Serine hydroxymethyltransferase (SHMT) reversibly interconverts serine and tetrahydrofolate (THF) into glycine and 5,10-methylene-THF (5,10-meTHF). Next, we have obtained high resolution crystal structures of AtSHMT2 complexed with MTX and PTX, as well as of AtSHMT4-MTX complex. For clarity, in this work we divide THF, MTX, and PTX molecules into three moieties: (i) pteridine or its mimic (P-moiety); (ii) benzoyl (B-moiety); and (iii) glutamate (E-moiety).

Soaking crystals of AtSHMT2 with PTX and serine revealed two distinct forms, resembling situation observed for AtSHMT2-MTX complex. External PLP-Ser aldimine state (EA-type) is seen in chains B and C (PTX was not placed in chain A as suggested by poor Polder map coefficients). Internal aldimine + free serine state (IA-type) is present in chain D. In the EA-type of binding (Chain B), a direct H-bond binds exocyclic N2 of PTX to backbone O of Leu172. Water-mediated interactions involve each of the five heteroatoms in the P-moiety. Importantly, there is no π-stacking interaction involving PTX. Hydrophobic environment is ensured mostly by side chains of Leu172, Leu178, and Ile189 adjacent to PTX B-moiety. The carboxyl group (at Cα) forms a salt bridge with Nζ of Lys187. In the IA-pose (Chain D), PTX forms fewer H-bonds. Another feature that likely explains higher inhibitory efficiency of PTX against SHMTs is that it is able to bind deeper inside the cavity.

>SNAEKSRSSWIKQLNASLDEIDPEVADIIELEKARQWKGFELIPSENFTSLSVMQAVGSVMTNKYSEGYPGARYYGGNEYIDMAETLCQKRALEAFQLDPSKWGVNVQSLSGSPANFQVYTALLKPHERIMALDLPHGGHLSHGYQTDTKKISAVSIFFETMPYRLDENTGYIDYDQLEKSAVLFRPKLIVAGASAYARLYDYARIRKVCNKQKAVMLADMAHISGLVAAGVIPSPFEYADVVTTTTHKSLRGPRGAMIFFRKGLKEINKQGKEVMYDYEDRINQAVFPGLQGGPHNHTITGLAVALKQARTPEYKAYQDQVLRNCSKFAETLLAKGYDLVSGGTDNHLVLVNLKNKGIDGSRVEKVLELVHIAANKNTVPGDVSAMVPGGIRMGTPALTSRGFIEEDFAKVAEYFDLAVKIALKIKAESQGTKLKDFVATMQSNEKLQSEMSKLREMVEEYAKQFPTIGFEKETMRYKE[4x]> GSHMELTPDQQTLLHFIMDSYNKQRMPQEITNKILKEAFSAEENFLILTEMATNHVQVLVEFTKKLPGFQTLDHEDQIALLKGSAVEAMFLRSAEIFNKKLPSGHSDLLEARIRNSGISDEYITPMFSFYKSIGELKMTQEEYALLTAIVILSPDRQYIKDREAVEKLQEPLLDVLQKLCKIHQPENPQHFACLLGRLTELRTFNHHHAEMLMSWRVNDHKFTPLLCEIWDVQ;> KDHQLLRYLLD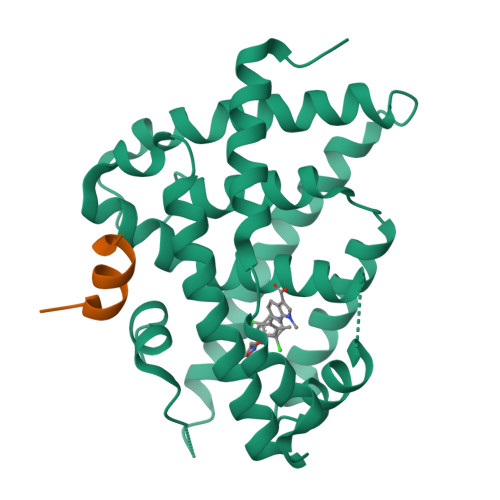KD>[4x]GSSSGQSNNNSDTCAEFRIKYVGAIEKLKLSEGKGLEGPLDLINYIDVAQQDGKLPFVPPEEEFIMGVSKYGIKVSTSDQYDVLHRHALYLIIRMVCYDDGLGAGKSLLALKTTDASNEEYSLWVYQCNSLEQAQAICKVLSTAFDSVLTSEKP;>[4x]GPLGSM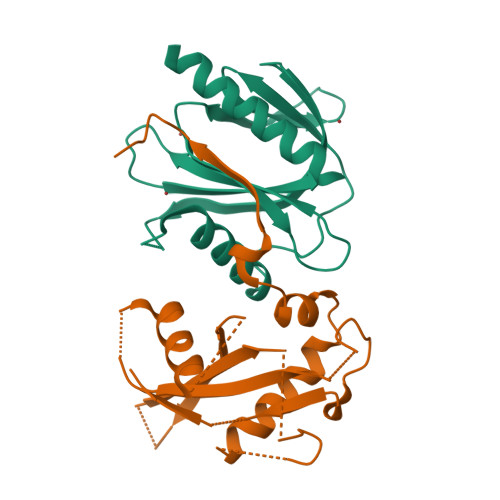GNPENIEDAYVAVIRPKNTASLNSREYRAKSYEILLHEVPIEGQKKKRKKVLLETKLQGNSEITQGILDYVVETTKPISPANQGIRGKRVVLMKKFPLDGEKMGREASLFIVPSVVKDNTKYTYTPGCPIFYCLQDIMRVCSESSTHFATLTARMLIALDKWLDERHAQSHFIPALFRPSPLERIKTNVINPAYATE>MKVRAQVPTVKNATNFNMVADSKTAVGSTLENLKAAIAGETGAHAKYTAFAKAAREQGYEQIARLFEATAAAELIHIGLEYALVAEMEPGYEKPTVAAPSAYSCDLNLISGANGEIYETSDMYPAFIRKAQEEGNSKAVHVFTRAKL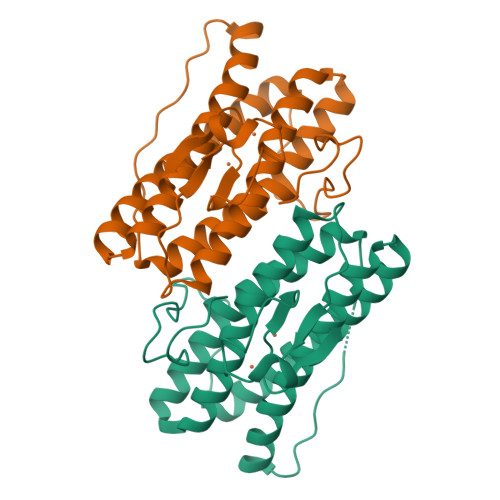AESVHAERYLAAYNDIDAPDDDKFHLCPICGYIHKGEDFEKCPICFRPKDTFTAY[2x]> SNAVQADYYQNMPGNNHTLAKEARSERGTIATYDGVVLARSVKEEDGTYEREYPAGDLASHVVGYSSPQFGNSGIEKAYNDTLKGEENFASWTDVLNSFAGIGTAGNDVTLTLNSKIQQAAQDALAGRKGACVVMDPDTGAILAMASAPTYNAADFAAVIEQANANPDDSTLVDRAAGSLYAPGSTFKIVTLATALEDDVAGEDTVFSSPGTMEIGNATVSNFNKANYGSLTLAQATELSSNTVFGQLGVEMGADKLVAGAESFGFNKEIDFPLYTPESLMPSAEDLQKSPWELAWAAAGEPVGDTTRPGRESPAGPQATVLEMAMVGTAIANDGVIMQPYLVDSVNNANGERSFSASPTKLMQAVSKTTAGRVRDVLLGVVQNGTGTAAAIPGIDVAGKTGTAEKENGNDSWFVGMAPAEDPRVVVAIVIEDGEEGVGTAKA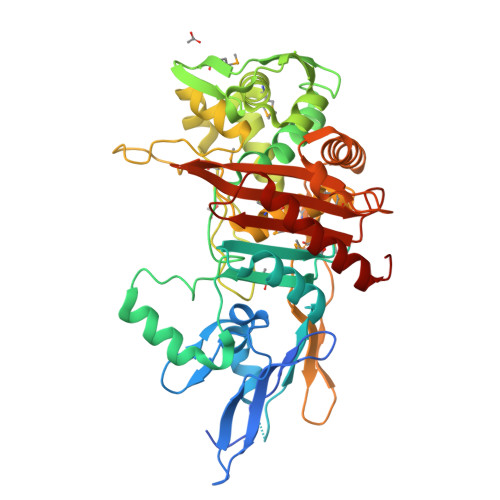QNVLKTALEVQGLL3-{2-deoxy-5-O-[(R)-hydroxy{[(R)-hydroxy(phosphonooxy)phosphoryl]oxy}phosphoryl]-beta-D-erythro-pentofuranosyl}-7-methyl-3H-imidazo[4,5-b]pyridine | C12 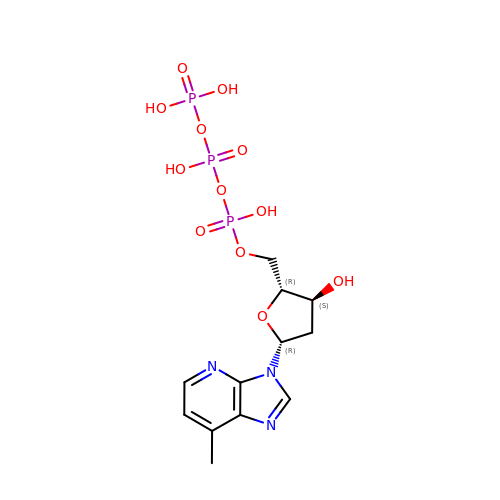H18 N3 O12 P3 | LSFMZRZQGVHWHK-IVZWLZJFSA-N>HMYYSYGNYEAFARPKKPENVENKSAYLIGSGLASLAAACFLIRDGQMEGSKIHILEELPKAGGSLDGENMPLKGYVVRGGREMENHFECLWDLFRSIPSLEIDNASVLDEFYWLNKEDPNYSRCRVIEKQGQRLVTDGDFTLTKTAIKEILDLCLTNEEDLDDVKITDVFSDDFFNSNFWIYWKTMFAFEPWHSAMEMRRYLMRFLHHISGLADFSALKFTKYNQYESLVLPMVEYLKSHGVQFEYDVKVEDIKIDVTTSQKIAREILIDRNGNAESIKLTINDLVFVTNGSITESSTYGDNDTPAPPTDELGGSWTLWKNLARQSPEFGNPDKFCQNIPKKSWFVSATSTTNNKEIIDTIESICKRDPLAGKTVTGGIITINDSAWQMSFTINRQQQFKDQPENEISTWIYALYSDVNGDYIKKPITECSGNEICQEWLYHLGVSTDKIEDLAKHASNTIPVYMPYITSYFMTRAIGDRPLVVPHQSQNLAFIGNFAETERDTVFTTEYSVRTAMEAVYQL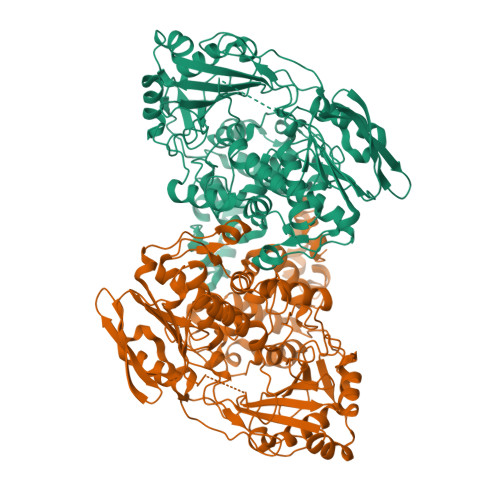LNIDRGIPEVINSPFDLRVLMDAIYELNDHQDLREITKDSKMQKLALAGFLKKIKGTYIESLLKEHKLL[3x]> GTELTDARRYWVDVTLATNNISHAVIAEDKRQV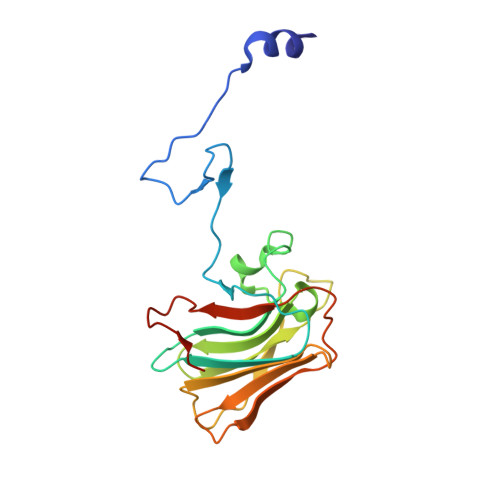SSRAGTGVLGSQSITSGKHYWEVDVSKKSAWILGVCAGFQSDAMYNIEQNENYQPKYGYWVIGLQEGVKYSVFQDGSSHTPFAPFIVPLSVIICPDRVGVFVDYEACTVSFFNITNHGFLIYKFSQCSFSKPVFPYLNPRKCTVPMTLCSPSS>[12x]SNAMSSEELEQVWSNIKSEARALAECEPMLASFFHATLLKHENLGSALSYILANKLANPIMPAIAIREVVEEAYRSDAHMIVSAARDILAVRLRDPAVDKYSTPLLYLKGFHALQAYRIGHWLWAQDRKALAIYLQNQVSVAFGVDIHPAATIGCGIMLDHATGIVIGETAVVENDVSILQSVTLGGTGKTSGDRHPK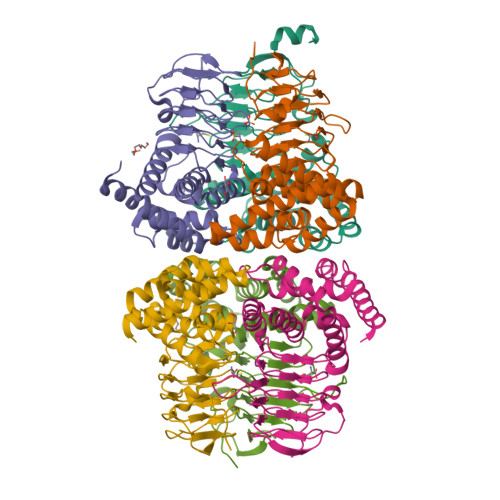IREGVMIGAGAKILGNIEVGRGAKIGAGSVVLQSVPAHTTAAGVPARIVGKPESDKPSLDMDQHFNGSIQGFEYGDGI>[4x]HHHHHHMALQLAAHSDARSGPVGSNGGQFWSFRPVRPLNKIVLSFSGSPDQTLNLISITFSSNPTDIITVGGV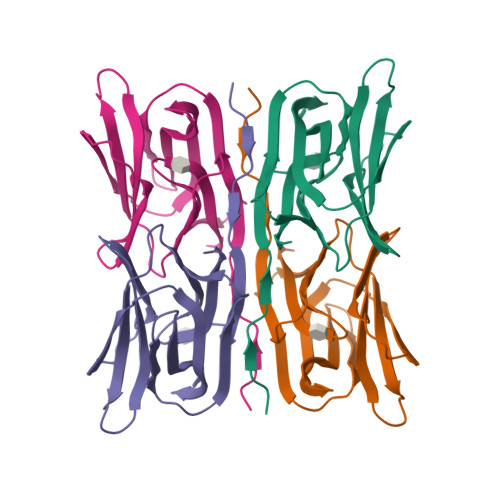GPEPLTYTETVNIDGDIIEISGMIANYKGYNVIRSIKFTTNKKEYGPYGANAGTPFNIKIPDGNKIVGFFGNSGWYVDAIGAYYTAK> RTIVVTTILESPYVMYKKNHEQLEGNERYEGYCVDLAYEIAKHVRIKYKLSIVGDGKYGARDPETKIWNGMVGELVYGRADIAVAPLTITLVREEVIDFSKPFMSLGISIMIKKGTPIESAEDLAKQTEIAYGTLASGSTKEFFRRSKIAVYEKMWSYMKSAEPSVFTKTTADGVARVRKSKGKFAFLL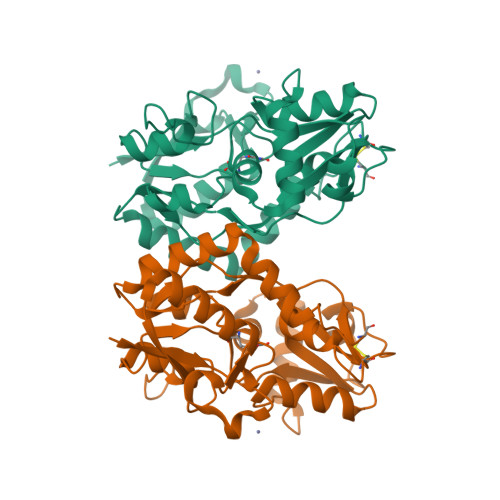ESTMNEYIEQRKPCDTMKVGGNLDSKGYGVATPKGSALGNAVNLAVLKLNEQGLLDKLKNKWWYDKGEC> MGSSHHHHHHHSQDPAEKQKHDGRVKIGHYVLGDTLGVGTFGKVKIGEHQLTGHKVAVKILNRQKIRSLDVVGKIKREIQNLKLFRHPHIIKLYQVISTPTDFFMVMEYVSGGELFDYICKHGRVEEMEARRLFQQILSAVDYCHRHMVVHRDLKPENVLLDAHMNAKIADFGLSNMMSDGEFLRTSCGSPNYAAPEVISGRLYAGPEVDIWSCGVILYALLCGTLPFDDEHVPTLFKKIRGGVFYIPEYLNRSVATLLMHMLQVDPLKRATIKDIREHEWFKQDLPSYLFPEDPSYDANVIDDEAVKEVCEKFECTESEVMNSLYSGDPQDQLAVAYHLIIDNRRIMNQASEFYLASSPPDSFLDDHHLTRPHPERVPFLVAETPRARHTLDELNPQKSKHQGVKKAKWHLGIRSQSKPYDIMAEVYRAMKQ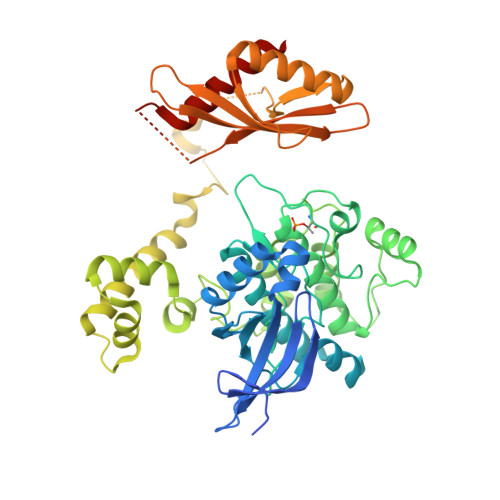LDFEWKVVNAYHLRVRRKNPVTGNYVKMSLQLYLVDNRSYLLDFKSIDDEVVEQRSGSSTPQRSCSAAGLHRPRSSFDSTTAESHSLSGSLTGSLTGSTLSSVSPRLGSHTMDFFEMCASLITTLAR> HVKSGLQIKKNAIIDDYKVTSQVLGLGINGKVLQIFNKRTQEKFALKMLQDCPKARREVELHWRASQCPHIVRIVDVYENLYAGRKCLLIVMECLDGGELFSRIQDRGDQAFTEREASEIMKSIGEAIQYLHSINIAHRDVKPENLLYTSKRPNAILKLTDFGFAKETTGHNSL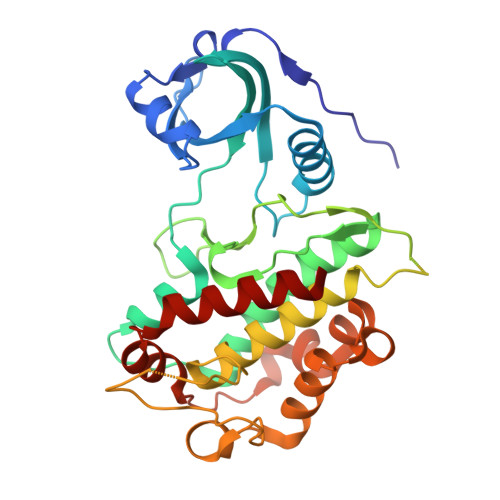TTPCYTPYYVAPEVLGPEKYDKSCDMWSLGVIMYILLCGYPPFYSNHGLAISPGMKTRIRMGQYEFPNPEWSEVSEEVKMLIRNLLKTEPTQRMTITEFMNHPWIMQSTKVPQTPLHTSRVLKEDKERWEDVKEEMTSALATMR The RNA polymerase complex of hPIV3, like other nsNSV members, consists of the large protein (L) and a co-factor protein, the phosphoprotein (P; or VP35 in the case of the filoviruses)4. L harbors five domains including the RNA dependent RNA polymerase (RdRp) domain, polyribonucleotidyltransferase (PRNTase) domain, connector domain (CD), methyltransferase (MTase) domain and the C-terminal domain (CTD), and possesses enzymatic activities required for RNA synthesis, cap addition and cap methylation. The P protein consists of an N-terminal domain (NTD), central oligomerization domain (OD) and C-terminal X domain (XD). Here, we report the cryo-electron microscopy (cryo-EM) structures of hPIV3 L–P polymerase in monomeric and incomplete dimeric forms.

We employed single-particle cryo-EM to solve the hPIV3 L–P complex structure at a high resolution up to 2.7 Å (class 1), allowing us to build a detailed atomic model. The overall structural architecture of hPIV3 L–P is similar to that of PIV56 and NDV L–P18, with corresponding sequence identities of 28% and 25%, respectively for L and both <10% for P. Interestingly, a large extra blob of electron density, not reported in previous L–P structures, was unambiguously observed near the intact L protein and was successfully assigned as the CD domain (named CD′) of a second L protein. In the hPIV3 L–P structure with CD′ of the second L, CD′ contacts the RdRp and PRNTase domains of the visible full L, with a large total buried interface of 2452 Å2 composed of electrostatic and hydrophobic interactions. At the interface, the charged residues Arg1509, Asp1510, Asp1576 and Glu1620 on CD′ form salt bridges with Glu1112, Arg1101, Arg1116 and Arg1119 on a long α-helix of PRNTase. In addition, Trp1513 of CD′ forms a cation–π interaction with Arg1101 of PRNTase. CD′ has nearly the same overall structure as the CD domain of the intact L, except for the two loops that contribute to the L–L interface and the bent helix α2 (Asp1430–Asp1456) of CD′. Interestingly, adopting such a bent α2 conformation could cause potential steric clashes for the interface between CD and RdRp-PRNTase within one L. The structure reveals that the two CD domains can exquisitely bind to distinct interfaces on RdRp and PRNTase domains, thus acting as both intramolecular and intermolecular connectors. Interestingly, CD′ is positioned adjacent to the putative template entry of the neighboring L and has a positively charged inner surface connected to the RNA tunnel, which suggests CD′ may provide a channel to transport RNA from polymerase into the adjoining polymerase. A triple mutant R1509A/D1510A/W1513A had a profound effect, reducing both antigenome and mRNA to almost undetectable levels. Here, the hPIV3 L–P dimer we captured appears to be asymmetric, otherwise serious steric clashes would be introduced between two L–P monomers.

>[2x]MISNQQSDNGQKENIKNLGAKRARKMDTESNNGTVSDILYPECHLNSPIVKGKIAQLHTIMSLPQPYDMDDDSILVITRQKIKLNKLDKRQRSIRRLKLILTEKVNDLGKYTFIRYPEMSKEMFKLYIPGINSKVTELLLKADRTYSQMTDGLRDLWINVLSKLASKNDGSNYDLNEEINNISKVHTTYKSDKWYNPFKTWFTIKYDMRRLQKARNEITFNVGKDYNLLEDQKNFLLIHPELVLILDKQNYNGYLITPELVLMYCDVVEGRWNISACAKLDPKLQSMYQKGNNLWEVIDKLFPIMGEKTFDVISLLEPLALSLIQTHDPVKQLRGAFLNHVLSEMELIFESGESIREFLSVDYIDKILDIFNESTIDEIAEIFSFFRTFGHPPLEASIAAEKVRKYMYIEKQLKFDTVNKCHAIFCTIIINGYRERHGGQWPPVTLPDHAHEFIINAYGSNSAISYENAVDYYQSFIGIKFNKFIEPQLDEDLTIYMKDKALSPKKSNWDTVYPASNLLYRTNASNESRRLVEVFIADSKFDPHQILDYVESGDWLDDPEFNISYSLKEKEIKQEGRLFAKMTYKMRATQVLSETLLANNIGKFFQENGMVKGEIELLKRLTTISISGVPRYNEVYNNSKSHTDDLKTYNKISNLNLSSNQKSKKFEFKSTDIYNDGYETVSCFLTTDLKKYCLNWRYESTALFGETCNQIFGLNKLFNWLHPRLEGSTIYVGDPYCPPSDKEHISLEDHPDSGFYVHNPRGGIEGFCQKLWTLISISAIHLAAVRIGVRVTAMVQGDNQAIAVTTRVPNNYDYRIKKEIVYKDVVRFFDSLREVMDDLGHELKLNETIISSKMFIYSKRIYYDGRILPQALKALSRCVFWSETVIDETRSASSNLATSFAKAIENGYSPVLGYACSIFKNIQQLYIALGMNINPTITQNIKDQYFKNSNWMQYASLIPASVGGFNYMAMSRCFVRNIGDPSVAALADIKRFIKANLLDRSVLYRIMNQEPGESSFLDWASDPYSCNLPQSQNITTMIKNITARNVLQDSPNPLLSGLFTNTMIEEDEELAEFLMDRKVILPRVAHDILDNSLTGIRNAIAGMLDTTKSLIRVGINRGGLTYSLLRKISNYDLVQYETLSRTLRLIVSDKIRYEDMCSVDLAIALRQKMWIHLSGGRMISGLETPDPLELLSGVVITGSEHCKICYSSDGTNPYTWMYLPGNIKIGSAETGVSSLRVPYFGSVTDERSEAQLGYIKNLSKPAKAAIRIAMIYTWAFGNDEISWMEASQIAQTRANFTLDSLKILTPVATSTNLSHRLKDTATQMKFSSTSLIRVSRFITMSNDNMSIKEANETKDTNLIYQQIMLTGLSVFEYLFRLKETTGHNPIVMHLHIEDECCIKESFNDEHINPESTLELIRYPESNEFIYDKDPLKDVDLSKLMVIKDHSYTIDMNYWDDTDIIHAISICTAITIADTMSQLDRDNLKEIIVIANDDDINSLITEFLTLDILVFLKTFGGLLVNQFAYTLYSLKIEGRDLIWDYIMRTLRDTSHSILKVLSNALSHPKVFKRFWDCGVLNPIYGPNTASQDQIKLALSICEYALDLFMREWLNGVSLEIYICDSDMEVANDRKQAFISRHLSFVCCLAEIASFGPNLLNLTYLERLDLLKQYLELNIKEDPTLKYVQISGLLIKSFPSTVTYVRKTAIKYLRIRGISPPEVIDDWDPIEDENMLDNIVKTINDNCNKDNKGNKINNFWGLALKNYQVLKIRSITSDSDDNDRLDASTSGLTLPQGGNYLSHQLRLFGINSTSCLKALELSQILMKEVNKDKDRLFLGEGAGAMLACYDATLGPAINYYNSGLNITDVIGQRELKIFPSEVSLVGKKLGNVTQILNRVKVLFNGNPNSTWIGNMECESLIWSELNDKSIGLVHCDMEGAIGKSEETVLHEHYSVIRITYLIGDDDVVLVSKIIPTITPNWSRILYLYKLYWKDVSIISLKTSNPASTELYLISKDAYCTIMEPSEVVLSKLKRLSLLEENNLLKWIILSKKRNNEWLHHEIKEGERDYGVMRPYHMALQIFGFQINLNHLAKEFLSTPDLTNINNIIQSFQRTIKDVLFEWINITHDDKRHKLGGRYNIFPLKNKGKLRLLSRRLVLSWISLSLSTRLLTGRFPDEKFEHRAQTGYVSLADTDLESLKLLSKNIIKNYRECIGSISYWFLTKEVKILMKLIGGAKLLGIPRQYKEPEEQLLENYNQHDEFDIDDYKDDDDK;>[5x]MESDAKNYQIMDSWEEESRDKSTNISSALNIIEFILSTDPQEDLSENDTINTRTQQLSATIYQPKIKPTETSEKDSGSTDKNRQSGSSHECTTEAKDRTIDQETVQRGPGRRSSSDSRAETVVSGGISRSITNSKNGTQNTEDIDLNEIRKMDKDSIEGKVRQSADVPSEISGSDVIFTTEQSRNSDHGRSLESISTPDTRSISVVTAATPDDEEEILMKNSRTKKSSSIHQEDDKRIKKGGKGKDWFKKSKDTDNQIPTSDYRSTSKGQKKISKTTTINTDTKGQTEIQTESSGTQSSSWNLTIDNNTDRTEQTNTTPPTTTSGSTYTKESIRTNSGSKPKTQKTNGKERKDTEESNRFTERAITLLQNLGVIQSTSKLDLYQDKRVVCVANVLNNVDTASKIDFLAGLVIGVSMDNDTKLTQIQNEMLNLKADLKKMDESHRRLIENQREQLSLITSLISNLKIMTERGGKKDQNESNERVSMIKTKLKEEKIKKTRFDPLMETQGIDKNIPDLYRHAGNTLENDVQVKSEILSSYNESNATRLIPKKVSSTMRSLVAVISNSNLSQSTKQSYINELKHCKNDEEVSELMDMFNEDVNNCQHHHHHH>MTNQKFFTLSNGNKIPAVAVVGVGTKWAHAEETDATFSQELTDIVKLSLDTVPGIVHIDAAEMYKTYPELGAALKETKKPREEIFITDKFSSLHKISEDPKSALETALNKLGVDYVDLYLIHSPFFDKDLNIDLETAWKQLEELYKSGKAKNIGVSNFTVEDLKKVLAIAEIKPQVNQIEFSPFLQNQTPGIVEFSQKNDILLEAYSPLGPLAKKPTD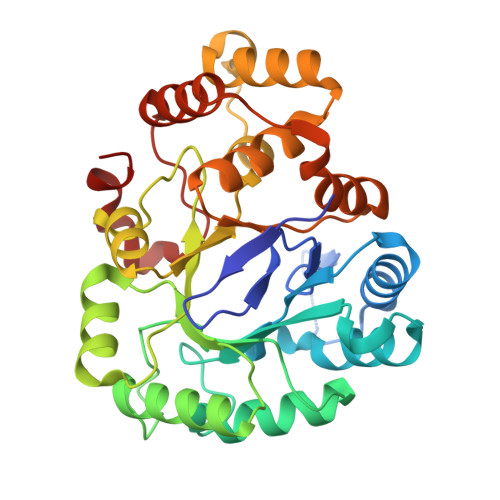ADQQPFYQYLKELSEKYNKTEAQVLLLWVYKRGILPVTTSAKIERIKQAQDIFSFDLTEEEVKKITDLGLQHEPVRLWHVDFYTKYNSEAQK[4x]> MVQDTGKDTNLKGTAEANESVVYCDVFMQAALKEA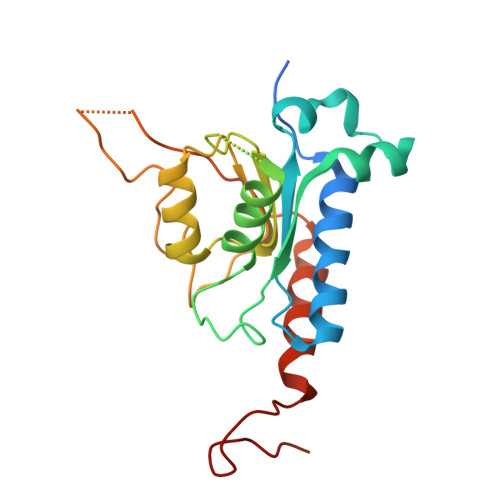TCALEEGEVPVGCVLVKADSSTAAQAQAGDDLALQKLIVARGRNATNRKGHGLAHAEFVAVEELLRQATAGTSENIGGGGNSGAVSQDLADYVLYVVVEPCIMCAAMLLYNRVRKVYFGCTNPRFGGNGTVLSVHNSYKGCSGEDAALIGYESCGGYRAEEAVVLLQQFYRRENTNAPLGKRKRKD>[2x]MSLDSISLIKTPIEAELEDFKALFDTPLSDSNALLDSVITHIRKRNGKMMRPILVLLVARL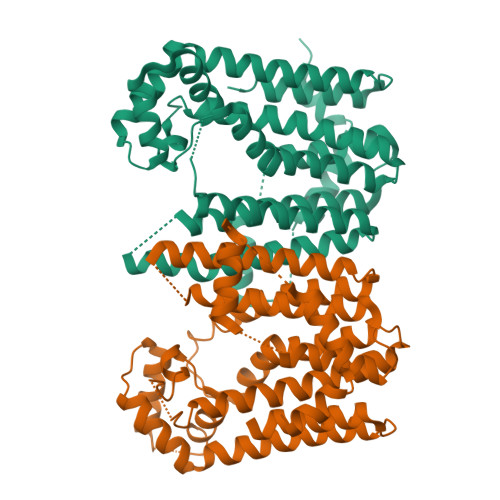YGAVTPATLHAAVSLELLHTASLVHDDVVDESTERRGQLSVNAIFNNKVSVLAGDYLLATSLVHAEQTNNYEIIRLVSSLGQKLAEGELLQLSNVSNHSFSEEVYFDVIRKKTAALFAACAEAAALSVQVGEEEVAFARLLGEYIGICFQIKDDIFDYFDSKKIGKPTGNDMLEGKLTLPALYALNTTKDAWAEQIAFKVKEGTATPDEIVRLIEFTKDNGGIEYACRTIEQYKKKAFDLLAALPDSNICLALRTYLDYVVAREKEGHHHHHH>C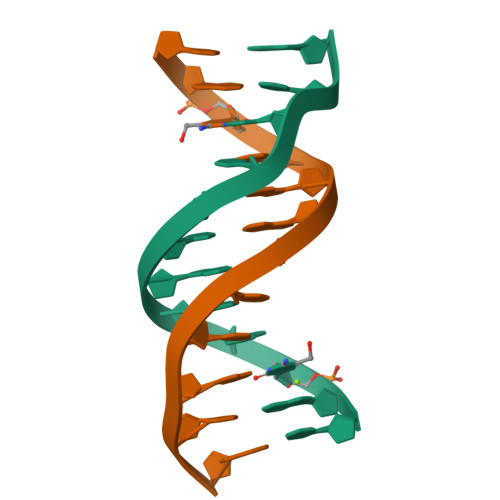GXGAATTCGCG[2x]> GSASQIVQNQSSLAPELSGCPPMGICMDGTIGDPI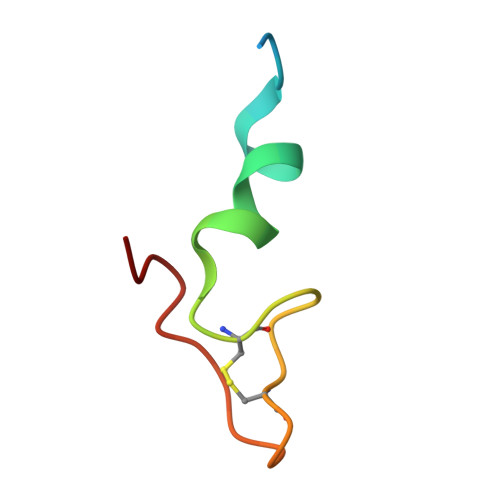AS DEAH-box adenosine triphosphatases (ATPases) play a crucial role in the spliceosome-mediated excision of pre-mRNA introns. The catalytic activation, the catalysis itself as well as the final disassembly steps are driven by so-called DEAH-box helicases. They all belong to the helicase superfamily 2 (SF2) and share at least eight conserved sequence motifs (motifs I, Ia, Ib, II, III, IV, V and VI) spread over two RecA-like domains that together form the helicase core. Two RecA-like domains, referred to as RecA1 and RecA2, build up the helicase core. The RecA2 domain contains an anti-parallel β-hairpin present in all DExH-box helicases, which protrudes out of the RecA2 domain thereby contacting the C-terminal domains. These domains are divided in three distinct domains, namely the winged-helix (WH), the helix-bundle (HB) and the oligonucleotide-binding (OB) domain.

For the crystallization of the complex structure of ctPrp22 with a single-stranded RNA, a U12-RNA was used, of which nine nucleotides were traceable in the electron density map. In the Prp22-RNA complex structure, the ssRNA is also predominantly bound via polar interactions with the sugar-phosphate backbone. The only exceptions are U9, as the base forms hydrogen-bond interactions with the side chains of N919 and R660, and the bases of U1-U3 that interact via π–π-stacking with F1134 and cation–π stacking with R1012. The thorough analysis of the Prp22–RNA complex structure reveals a novel RNA-binding motif present in the OB-fold domain, which involves H1128, P1129 and F1134 as a stacking triad. H1128 directly interacts via hydrogen-bonding with the phosphate of U4 and the ribose of U3, but also undergoes stacking with P1129, which itself stacks with F1134. This last residue of the stacking triad π–π-stacks in a parallel-displaced manner with the U1 base as well as in an edge-to-face fashion with the U2 base. All these interactions lock the 5′ end of the RNA into a conformation where the bases point into the opposite direction of the β-hairpin of the RecA2 domain. The presence of ADP/ATP seems to stabilize closed conformations of the helicase core regardless of the availability of RNA, while in the absence of adenosine nucleotides the bound RNA suppresses the mobility of the RecA2 domain and stabilizes the helicase core in an open conformation with a RecA1-RecA2 center of mass distance of 31.7 Å. B-factor values of the RecA2 domain are not elevated anymore in the Prp22–RNA complex structure. While the DEAH-box ATPase encloses a stack of four RNA nucleotides in the closed and ATP-bound state, this open and adenosine nucleotide-free conformation accommodates a five-nucleotide stack in the RNA-binding tunnel.

>[4x]TNMSIKEQRESLPVFQFRDQIIQAVKDNQILIVVGETGSGKTTQVTQYLAEAGFTKYGMIGCTQPRRVAAVSVAKRVAEEVGCQLGQEVGYTIRFEDVTSPATKIKYMTDGMLQREILMDPDLKRYSVIMLDEAHERTIATDVLFALLKKTVKRRPDLKVIVTSATLDAEKFSEYFNSCPIFTIPGRTFPVEILYSREPEPDYLEAALTTVMQIHLTEPPGDILVFLTGQEEIDTACEILYERMKALGPSVPELIILPIYSALPSEMQSRIFEPAPPGSRKVVIATNIAETSITIDYIYYVVDPGFVKQNAYDPKLGMDSLVVTPISQAQANQRAGRAGRTGPGKCFRLYTEAAYQSEMLPTTIPDIQRQNLANTILLLKAMGINDLLRFDFMDPPPVNTMLTALEELYALGALDDEGLLTRLGRKMADFPMEPSLSKVLIASVDKGCSDEMVTIVSMLNLQQIFYRPKDKQQQADQKKAKFHDPTGDHLTLLNVYNAWKNSGYSNAWCFENYIQARAMRRARDVRQQIVKIMERHRHPIISCGRDTDKIRQALCAGFFRNTARKDPQEGYKTLTEGTPVYLHPSSALFGKQAEWVLYHELVLTTKEYMHFTTAIEPKWLVEAAPTFFKLAPTDRLSKRKKAERIQPLYNKYEGEDGWRLSAQRRAARPGGGGGTWG> PISPIETVPVKLKPGMDGPKVKQWPLTEEKIKALVEICTEMEKEGKISKIGPENPYNTPVFAIKKKDSTKWRKLVDFRELNKRTQDFWEVQLGIPHPAGLKKKKSVTVLDVGDAYFSVPLDEDFRKYTAFTIPSINNETPGIRYQYNVLPQGWKGSPAIFQSSMTKILEPFRKQNPDIVICQYMDDLYVGSDLEIGQHRTKIEELRQHLLRWGLTTPDKKHQKEPPFLWMGYELHPDKWTVQPIVLPEKDSWTVNDIQKLVGKLNWASQIYPGIKVRQLCKLLRGTKALTEVIPLTEEAELELAENREILKEPVHGVYYDPSKDLIAEIQKQGQGQWTYQIYQEPFKNLKTGKYARMRGAHTNDVKQLTEAVQKITTESIVI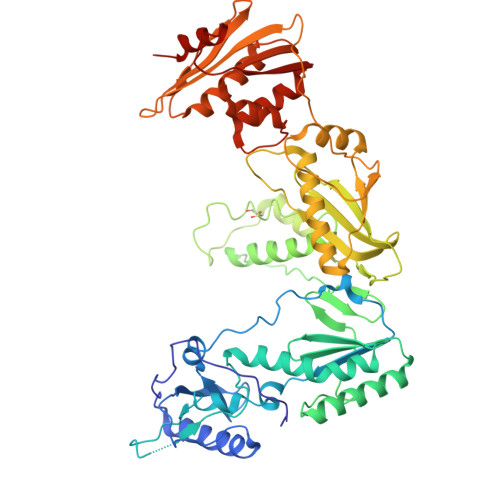WGKTPKFKLPIQKETWETWWTEYWQATWIPEWEFVNTPPLVKLWYQLEKEPIVGAETFYVDGAANRETKLGKAGYVTNRGRQKVVTLTDTTNQKTELQAIYLALQDSGLEVNIVTDSQYALGIIQAQPDQSESELVNQIIEQLIKKEKVYLAWVPAHKGIGGNEQVDKLVSAGIRKVL>[2x]MELESSERELIAAEAQR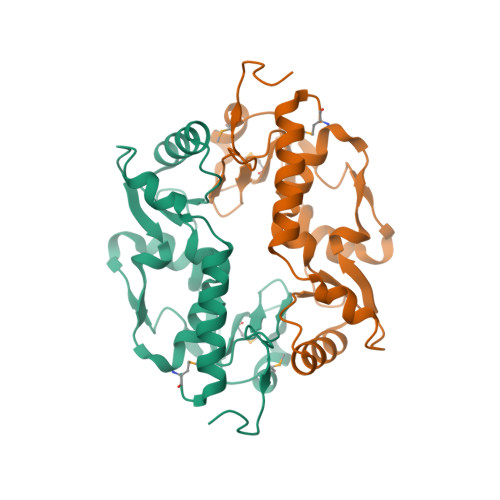EVRGNRAAEELKRSGIGGIYGTLAELIKVKDEAYALAIEVALGNRADNVVVEDELVAEKAIKYLKEHKLGRLTFLPLNKIKPKHVDSSVGLPAVDVIEYDQKIENAVKFALGDTVIVNSMEEARPHIGKVRMVTIEGELYERSGAITGGHFRARGLAVDTTKLRLEHHHHHH>[4x]MQKQRTTSQWRELDAAHHLHPFTDTASLNQAGARVMTRGEGVYLWDSEGNKIIDGMAGLWCVNVGYGRKDFAEAARRQMEELPFYNTFFKTTHPAVVELSSLLAEVTPAGFDRVFYTNSG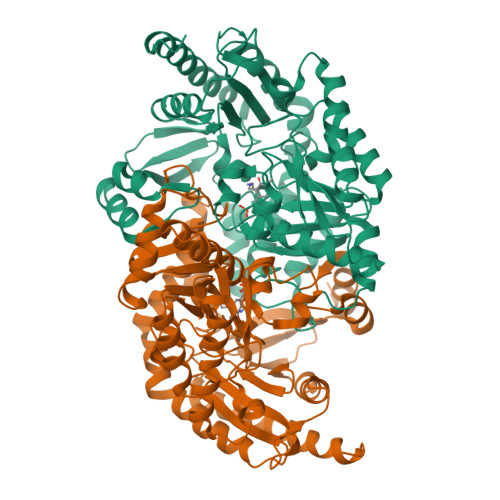SESVDTMIRMVRRYWDVQGKPEKKTLIGRWNGYHGSTIGGASLGGMKYMHEQGDLPIPGMAHIEQPWWYKHGKDMTPDEFGVVAARWLEEKILEIGADKVAAFVGEPIQGAGGVIVPPATYWPEIERICRKYDVLLVADEVICGFGRTGEWFGHQHFGFQPDLFTAAKGLSSGYLPIGAVFVGKRVAEGLIAGGDFNHGFTYSGHPVCAAVAHANVAALRDEGIVQRVKDDIGPYMQKRWRETFSRFEHVDDVRGVGMVQAFTLVKNKAKRELFPDFGEIGTLCRDIFFRNNLIMRACGDHIVSAPPLVMTRAEVDEMLAVAERCLEEFEQTLKARGLA> MARVGPGRAGVSCQGRGRGRGGSGQRRPPTWEISDSDAEDSAGSEAAARARDPAGERRAAAEALRLLRPEQVLKRLAVCVDTAILEDAGADVLMEALEALGCECRIEPQRPARSLRWTRASPDPCPRSLPPEVWAAGEQELLLLLEP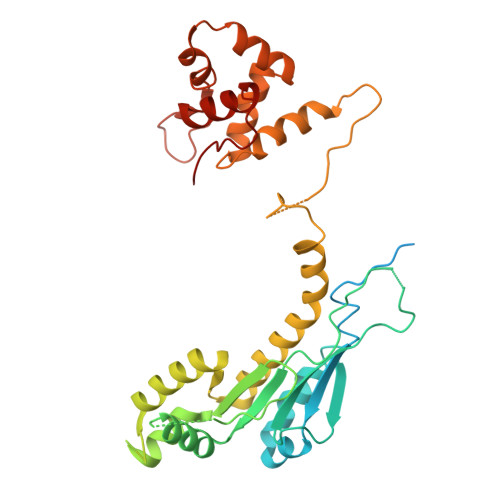EEFLQGVATLTQISGPTHWVPWISPETTARPHLAVIGLDAYLWSRQHVSRGTQQPESPKVAGAEVAVSWPEVEEALVLLQLWANLDVLLVASWQELSRHVCAVTKALAQYPLKQYRESQAFSFCTAGRWAAGEPVARDGAGLQAAWRRQIRQFSRVSPAVADAVVTAFPSPRLLQQALEACSTERERMGLLADLPVPPSEGGRPRRVGPDLSRRICLFLTTANPDLLLDLGS(2R,3S,5R,7S)-2-(pyridin-3-yl)-1-azatricyclo[3.3.1.1~3,7~]decane | C14 H18 N2 | 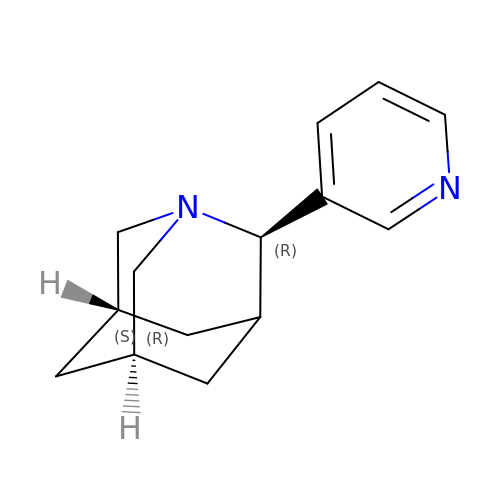INDYXBQOPZTSTJ-XCCSTKFXSA-N>SNAMKTVTVRDLVVGEGAPKIIVSLMGKTITDVKSEALAYREADFDILEWRVDHFANVTTAESVLEAAGAIREIITDKPLLFTFRSAKEGGEQALTTGQYIDLNRAAVDSGL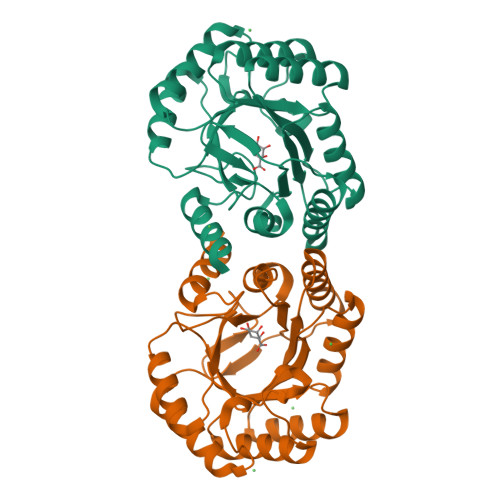VDMIDLELFTGDDEVKATVGYAHQHNVAVIMSNHDFHKTPAAEEIVQRLRKMQELGADIPKIAVMPQTKADVLTLLTATVEMQERYADRPIITMSMSKTGVISRLAGEVFGSAATFGAVKKASAPGQISVADLRTVLTILHQA[2x]>MKKWLYIFILFLVAGLGSTSSADAKMPGEKSVNVSKLNVDEFFKDRDGTFILHDVQKDKTFIYNESRAKERQTPQSTFKVPNALIGLQVKAVRDEYDVKRWDGTEREFESWNRDHTLGSAMRDSVIWYYQAMARDIGEDRMKDWLHRISYGNEDISGGIDQFWLQSSLKISPLEEKDFIEHLYKEDLPFDKPIMKTVKRMMIQEEGDHYTLYGKTGTRLTDYGLGWFVGFITTDNHSYIFVTNVDASGTAAKNI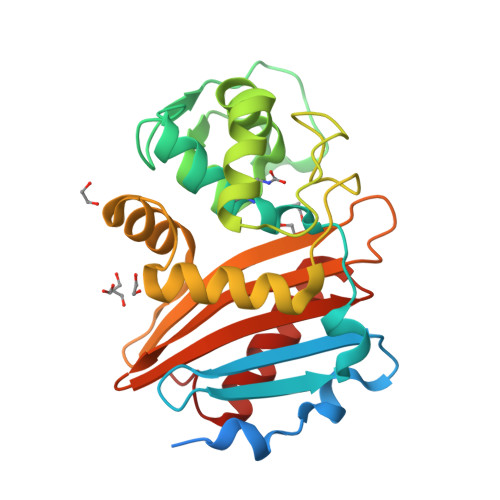TTDILKKYHLITN[2x]2-(2-amino-1H-1,3-benzimidazol-4-yl)-N-{4-[(pyridin-4-yl)methyl]phenyl}acetamide 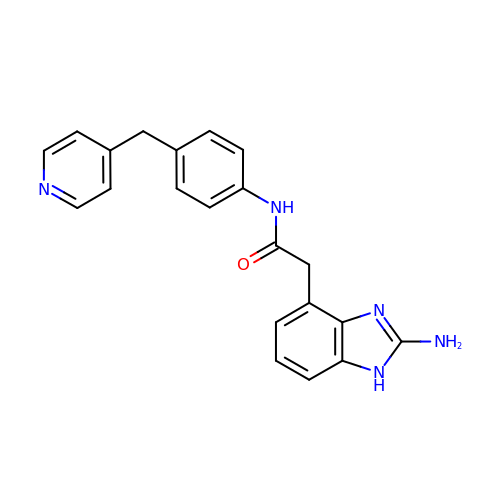| C21 H19 N5 O | AGVCSHCLKHPSSZ-UHFFFAOYSA-N> QPPLAPGLSFDFYKRSCPKAESIVRSFVQDAVRRDVGLAAGLLRLHFHDCFVQGCDASVLLDGSATGPGEQQAPPNLTLRPTAFKAINDIHDRLHKECGGTVVSCSDVLALAARDSVVVSGGPSYRVPLGRRDSASFATQQDVLSGLPPPTAAVPALLAVLSKINLDATDLVALSGGHTIGLGHCTSFEDRLFPRPDPTLNATFAGQLRRTCPAKGTDRRTPLDVRTPNAFDNKYYVNLVNREGLFTSDQDLFSNARTRALVDKFARSQRDFFDQFAFSVVKMGQIKVLTGTQGQIRTNCSARNAAG

We have purified pure cationic sorghum peroxidase from the Nigerian Sorghum grain variety SK 5912. The purification profile, using cation exchange chromatography, revealed a single basic peroxidase, similar to that previously reported for a related sorghum peroxidase. SK 5912 sorghum peroxidase shows a high degree of sequence identity to other class III plant peroxidases, Figure S1. The overall structure contains 306 residues and closely resembles the structures of other class III peroxidases—namely barley peroxidase (BP1), with an RMSD of 0.652 over 306 Cα atoms, as well as peanut peroxidase (PNP) and horseradish peroxidase (HRP). The class III heme peroxidases share common structural features, including four conserved disulphide bridges which are also observed in the sorghum enzyme (C50–C131, C83–C88, C138–C333 and C218–C245).

A notable difference between the typical class III peroxidases (HRP, PNP) and the sorghum enzyme is the position of the distal histidine: His 81 in the sorghum enzyme is much further from the iron (Nδ1 to Fe distance = 8.16 Å, compared to 5.9 Å in HRP). In the sorghum structure, a water molecule (W83) is found in the region that is occupied by the distal histidine in both HRP and PNP, and this water forms a hydrogen bond (2.75 Å) to Nδ1 of His81. Since the SK 5912 sorghum peroxidase is isolated from source (i.e. directly from the sorghum grains), we suggest that this IAA binds to the enzyme and is carried through the isolation and purification process. The class III heme peroxidases typically contain two calcium binding sites. In the sorghum structure there are also two metal ions, and at the same locations as found in HRP and PNP, Fig. 5a, d; in the sorghum structure, these are assigned as Na+ (on the distal side) and Ca2+ (on the proximal side) binding sites based on the ligand coordination geometries. The presence of Ca2+ and Na+ ions at these sites is consistent with the Ca2+-dependence of the steady state and pre-steady state kinetics above. It is probably the case that the catalytic activity of the sorghum enzyme is dependent on metal ion incorporation at these positions, or even that the activity is dependent on replacement of the distal sodium site with calcium (which would account for the calcium activation).The YTH (YT521-B homology) domain-containing proteins are a family of RNA-binding proteins that specifically recognize N 6-methyladenosine (m6A), the most abundant internal modification in eukaryotic RNA. In contrast, the DF proteins (DF1, DF2, and DF3) are mainly cytoplasmic and play essential roles in mRNA translation, stability, and degradation. Our study focuses on DF2, which is involved in multiple types of cancer, including prostate cancer, MYC-driven breast cancer, and acute myeloid leukemia (AML). We have also presented the crystal structures of DF2 in complex with six ligands, which represent six distinct chemotypes (compounds 3–6, 13, and 15).

The X-ray crystal structure was solved for compounds 3–6 at high resolution. In our first screening campaign, we described a series of uracil analogues; compound 4 is a new member of this series with a modest IC50 value of 250 μM. The six binders 1–6 belong to four distinct chemotypes: thiobarbiturates (1–3), uracil, nicotinamide, and pyrazolopyrimidine. Despite their chemical diversity, these chemotypes feature an NH group that is involved as a hydrogen-bond donor with the backbone carbonyl of C433. Furthermore, they act as hydrogen-bond acceptor of the conserved water that forms hydrogen bonds with the side chains of W432 and D528. Notably, compounds 1–3 occupy the bottom of the aromatic cage with their sulfur atom, while compounds 4–6 have a methyl group as in the natural ligand. Compounds 1–4 and 6 act as hydrogen-bond acceptors for the backbone NH of Y418, and they also form a hydrogen bond with the side chain of D422. This interaction may offer selectivity against the nuclear reader DC1, which features the N367 hydrogen-bond donor NH2 in this position.

>MGSSYHHHHHHSSGENLYFQHMKHGRVFIIKSYSEDDIHRSIKYNIWCSTEHGNKRLDAAYRSMNGKGPVYLLFSVNGSGHFCGVAEMKSAVDYNTCAGVWSQDKWKGRFDVRWIFVKDVPNSQLRHIRLENNENKPVTNSRDTQEVPLEKAKQVLKIIASYKHTTS[2x]TOPBP1 and its fission and budding yeast orthologues Rad4 and Dpb11, respectively, are scaffold proteins that mediate formation of multi-protein complexes in a range of essential DNA replication and repair processes. Bioinformatic analysis suggests that only three of the BRCT domains in the yeast TOPBP1 homologues, and four in the vertebrate TOPBP1 homologues, possess the required cluster of residues needed to bind phosphorylated peptide motifs. Despite the structural similarity of these phosphopeptide-binding BRCT domains, genetic and biochemical studies show that they are nonetheless selective and specific for the phosphopeptide sequences with which they interact. To gain some insight into this, we have determined crystal structures of segments of yeast and vertebrate TOPBP1 that contain the two most N-terminal phosphopeptide binding sites (BRCT1 and BRCT2), in complex with phosphopeptides derived from a number of different known ligand proteins, including RAD9, and used this to develop consensus patterns that encapsulate the individual specificity requirements of these two independent binding sites.

Phosphorylation of RAD9 on Ser387 (or its equivalent) in its C-terminal ‘tail’ has been shown to be essential for interaction with TOPBP1, and required for an effective checkpoint response in a Xenopus system. We have now succeeded in determining the crystal structure of the BRCT0,1,2 module of chicken TOPBP1 (cTOPBP1) in complex with a peptide corresponding to the phosphorylated C-terminus of human RAD9 at a resolution of 2.3 Å. As determined by mutagenesis studies, the RAD9-pS387 peptide binds to the middle BRCT domain (BRCT1) of the closely packed array that forms the N-terminus of cTOPBP1. Unlike phospho-peptide binding to the more commonly occurring C-terminal tandem BRCT2 arrangements where the bound peptide bridges consecutive BRCT domains, the RAD9-pS387 peptide runs perpendicular to the long axis of the BRCT-domain ‘array’ and only contacts BRCT1. The phosphate group of RAD9-pSer387 is recognised by a network of hydrogen bonding and ionic interactions centred around the side chains of cTOPBP1 residues Thr114, Arg121 and Lys155, which form the conserved triplet common to all BRCT-domains involved in binding phosphorylated peptide motifs. In addition to these core polar interactions with the phosphate, the side chain of RAD9-Asp386 hydrogen bonds to the side chain of cTOPBP1-Lys118. Upstream of pSer387 and Asp386 (−1, relative to phosphorylated residue), the peptide backbone of the RAD9 peptide main chain forms a distorted anti-parallel β-sheet with the main chain of a loop connecting cTOPBP1 residues 137 – 141, with an additional interaction between the side chain of cTOPBP1-Asp138 and the peptide nitrogen of RAD9-Asp386.

> RMKGSKEVFLVKFVKSSGSSEYFLKALESIKEFQSEEHLQILEEEAALNIKENDKSLYICDPFTGVVFNHLKKLGCRIVGPQVVLYCMQSQRCVPRAEYPVYNMTMADVTISCTTLDKDVREEVHKYVQMMGGRVYRDLNMSVTHLIAGEVGSKKYLVAASLKKPVLLPSWVKTLWDKSQQRMMRYTDVNMEDYACPVFLGCTICVTGLSSSDRKEVQRLTAEHGGQYSGQLKMNECTHLIVQEPKGQKYECAKKWNVHCVPVQWFSDSIEKGFCQDETMYKIESGSKLS;> SPVLAEDSEGE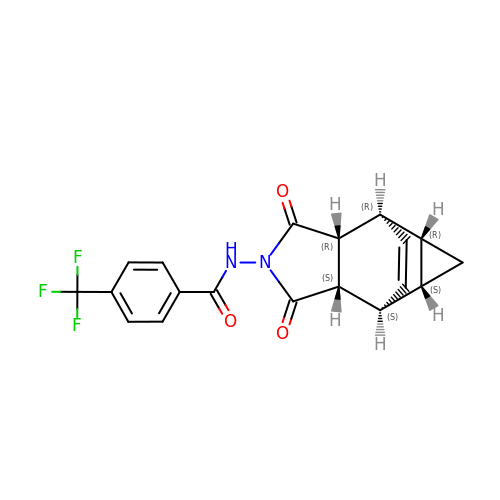Tecovirimat | C19 H15 F3 N2 O3 | CSKDFZIMJXRJGH-UHFFFAOYSA-N>[2x]GSHMKNSVSVDLPGSMKVLVSKSSNADGKYDLIATVDALELSGTSDKNNGSGVLEGVKADASKVKLTISDDLGQTTLEVFKSDGSTLVSKKVTSKDKSSTYELFNEKGELSAKYITRADKSSTYELF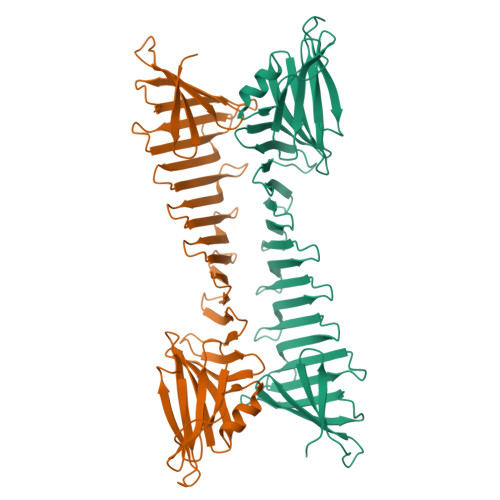NEKGELSFKYITRADKSSTYELFNEKGELSAKYITRADKSSTYELFNEKGELSAKYITRADGTRLEYTGIKSDGSGKAKEVLKGYVLEGTLTAEKTTLVVKEGTVTLSKNISKSGEVSVELNDTDSSAATKKTAAWNSGTSTLTITVNSKKTKDLVFTSSNTITVQQYDSNGTSLEGSAVEITKLDEIKNALK> NPKGW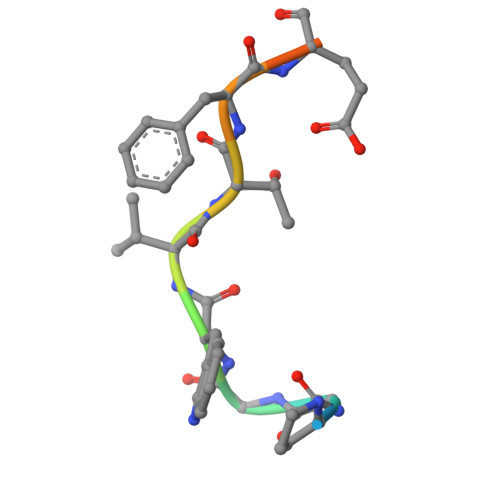VTFEEEE>EFHMTPEGLSSEQQRAFLAVTQTPHPAHLITGPAGTGKTTLLYALQKFYKGRAVTLAPTGTAALQARGQTVHSFFRFPARLLRYRHPEDIRPPGPHSPLRKAIEQMEVLILDEVGMVRVDLLEAMDWALRKTRKRLEEPFGGVKVLLLGDTRQLEPVVPGGEEALYIART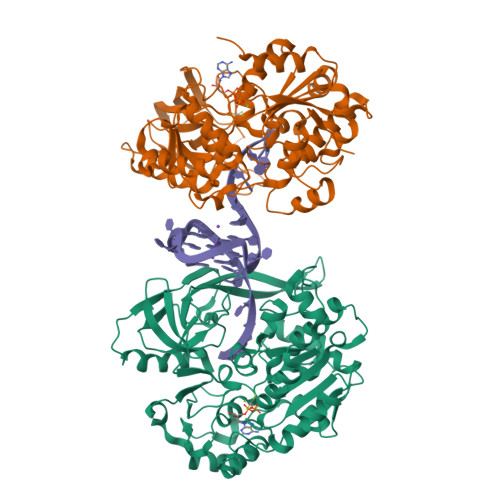WGGPFFFQAHVWEEVALRVHRLWESQRQREDPLFAELLKRLRQGDPQALETLNRAAVRPDGGEEPGTLILTPRRKEADALNLKRLEALPGKPLEYQAQVKGEFAETDFPTEAALTLKKGAQVILLRNDPLGEYFNGDLGWVEDLEAEALAVRLKRNGRRVVIRPFVWEKIVYTYDSEREEIKPQVVGTFRQVPVRLAWALTVHKAQGLTLDKVHLELGRGLFAHGQLYVALTRVRRLQDLSLSRPIAPTELLWRPEVEVFETRIQEGIWQKSHGWPSLVD[2x]> MSQPQSSQVTKRGLTDPERAAIIAAAVPDHALDTQRKYHYFIQPRWKPLSEYEQLSCYAQPNPDWIAGGLDWGDWTQKFHGGRPSWGNESTELRTTDWYRHRDPARRWHHPYVKDKSEEARYTQRFLAAYSSEGSIRTIDPYWRDEILNKYFGALLYSEYGLFNAHSSVGRDCLSDTIRQTAVFAALDKVDNAQMIQMERLFIAKLVPGFDASTDVPKKIWTTDPIYSGARATVQEIWQGVQDWNEILWAGHAVYDATFGQFARREFFQRLATVYGDTLTPFFTAQSQTYFQTTRGAIDDLFVYCLANDSEFGAHNRTFLNAWTEHYLASSVAALKDFVGLYAKVEKVAGATDSAGVSEALQRVFGDWKIDYADKIGFRVDVDQKVDAVLAGYKN;> MAISLATKAATNRAPVGVEPQEVHKWLQSFNWDFKENRTKYPTKYHMANETKEQFKVIAKEYARMEAAKDERQFGTLLDGLTRLGAGNKVHPRWGETMKVISNFLEVGEYNAIAASAMLWDSATAAEQKNGYLAQVLDEIRHTHQCAFINHYYSKHYHDPAGHNDARRTRAIGPLWKGMKRVFADGFISGDA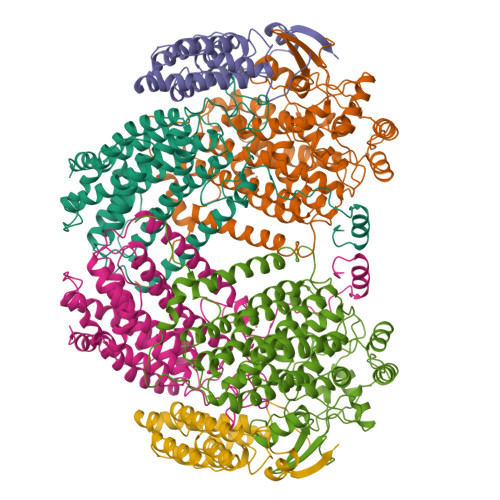VECSVNLQLVGEACFTNPLIVAVTEWASANGDEITPTVFLSVETDELRHMANGYQTVVSIANDPASAKFLNTDLNNAFWTQQKYFTPVLGYLFEYGSKFKVEPWVKTWNRWVSEDWGGIWIGRLGKYGVESPRSLRDAKRDAYWAHHDLALAAYAMWPLGFARLALPDEEDQAWFEANYPGWADHYGKIFNEWKKLGYEDPKSGFIPYQWLLANGHDVYIDRVSQVPFIPSLAKGTGSLRVHEFNGKKHSLTDDWGERQWLIEPERYECHNVFEQYEGRELSEVIAEGHGVRSDGKTLIAQPHTRGDNLWTLEDIKRAGCVFPDPLAKF;> MAKREPIHDNSIRTEWEAKIAKLTSVDQATKFIQDFRLAYTSPFRKSYDIDVDYQYIERKIEEKLSVLKTEKLPVADLITKATTGEDAAAVEATWIAKIKAAKSKYEAEAIHIEFRQLYKPPVLPVNVFLRTDAALGTVLMEIRNTDYYGTPLEGLRKERGVKVLHLQA> ACCGCCGGCGCC;> GGCGCCGG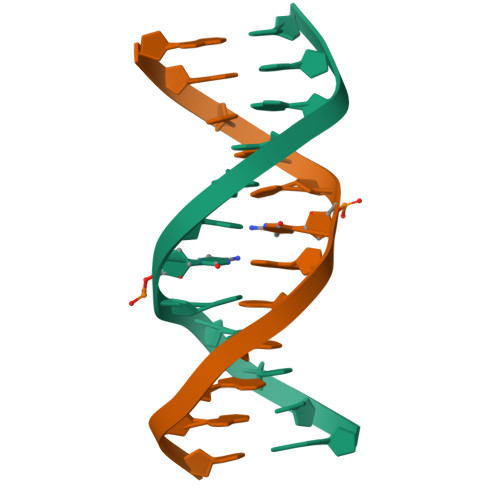CGGT>[2x]MKVQYCDSLVIGGGLAGLRAAVATQQKGLSTIVLSLIPVKRSHSAAAQGGMQASLGNSKMSDGDNEDLHFMDTVKGSDWGCDQKVARMFVNTAPKAIRELAAWGVPWTRIHKGDRMAIINAQKTTITEEDFRHGLIHSRDFGGTKKWRTCYTADATGHTMLFAVANECLKLGVSIQDRKEAIALIHQDGKCYGAVVRDLVTGDIIAYVAKGTLIATGGYGRIYKNTTNAVVCEGTGTAIALETGIAQLGNMEAVQFHPTPLFPSGILLTEGCRGDGGILRDVDGHRFMPDYEPEKKELASRDVVSRRMIEHIRKGKGVQSPYGQHLWLDISILGRKHIETNLRDVQEICEYFAGIDPAEKWAPVLPMQHYSMGGIRTDYRGEAKLKGLFSAGEAACWDMHGFNRLGGNSVSEAVVAGMIVGEYFAEHCANTQVDLETKTLEKFVKGQEAYMKSLVESKGTEDVFKIKNRMKDVMDDNVGIFRDGPHLEKSVKELEELYKKSKNVGIKNKRLHANPELEEAYRVPMMLKVALCVAKGALDRTESRGAHNREDYPKRDDINWLNRTLASWPNPEQTLPTLEYEALDVNEMEIAPRYRGYGAKGNYIENPLSVKRQEEIDKIQSELEAAGKDRHAIQEALMPYELPAKYKARNERLGDK;>[2x]MGRMLTIRVFKYDPQSAVSKPHFQEYKIEEAPSMTIFIVLNMIRETYDP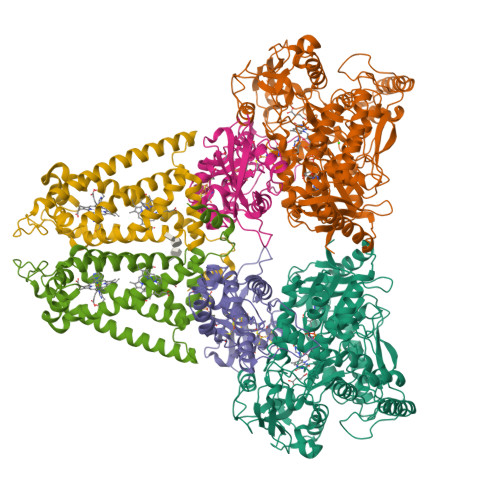DLNFDFVCRAGICGSCGMMINGRPSLACRTLTKDFEDGVITLLPLPAFKLIKDLSVDTGNWFNGMSQRVESWIHAQKEHDISKLEERIEPEVAQEVFELDRCIECGCCIAACGTKIMREDFVGAAGLNRVVRFMIDPHDERTDEDYYELIGDDDGVFGCMTLLACHDVCPKNLPLQSKIAYLRRKMVSVN;>[2x]MTNESILESYSGVTPERKKSRMPAKLDWWQSATGLFLGLFMIGHMFFVSTILLGDNVMLWVTKKFELDFIFEGGKPIVVSFLAAFVFAVFIAHAFLAMRKFPINYRQYLTFKTHKDLMRHGDTTLWWIQAMTGFAMFFLGSVHLYIMMTQPQTIGPVSSSFRMVSEWMWPLYLVLLFAVELHGSVGLYRLAVKWGWFDGETPDKTRANLKKLKTLMSAFLIVLGLLTFGAYVKKGLEQTDPNIDYKYFDYKRTHHR>[2x]GSGMGRRKKMVERVTTLMDKPEFIRNIGIVAHIDHGKTTLSDNLLAGAGMISKELAGEQLFMDFDEEEQKRGITIDSANVSMVHEYEGKEYLINLIDTPGHVDFGGDVTRAMRAVDGAVVVVDAVEGAMPQTETVLRQALRENVVPILFINKVDRLIMELKLTPQDMQIRLGAVIDKINKLIKGMKPDSYDGLRLDAAVGKVAFGSALNNWAISVPFMKKTGIGFKEVIEYCMEDQQQKLAERCPLHAVVNDMVIRFLPNPVQAQKERIKVIWHGDKGSEIG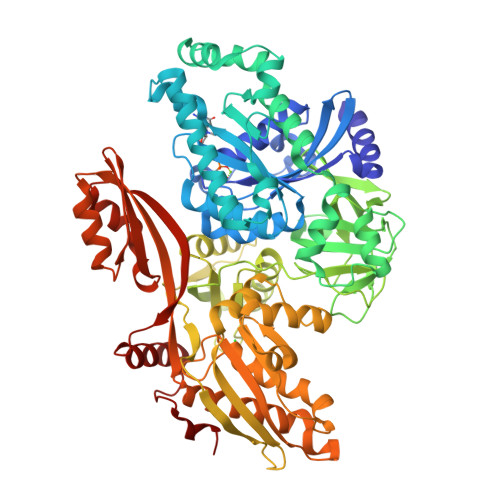KSMANVDPNGKVALMITDISTDPHAGEVATGRLFSGTLERGKEVYISGMPNPNRIQQVGLFMGPERIEVDRITAGNIVAVTGLADAIVGSTASTDKAMVPFESIRHVSEPVVTVAVEAKHMKDLPKLVEVLRQVAKEDPTLKVTINQETGEHLLAGMGELHLEIVAHRIQRDKHVEITTSKPLVVYRETVSAHAGPVEGKSPNRHNRFYIEIEPLQPAIFELVRNGEISMKQQEVERRDILMKAGMSKEEAKGITHISENNIFIDMTKGIQYLNETMELVLEGFEEVIKGGPLSREPVMGLKVKLMDAKLHEDSIHRGPAQVIPASRQAIQAAMLMAGATLLEPFQKVFIHVPQEQMGGAMREIQGRRGAILDMKTEGDTTIIEAKAPVAQLFGFAGDIRSATEGRAMWSTEFLGFEPIPANMLAETVMGIRQRKGLKLEMPKPSDFISP>GMQDERWNHPLYTTTAINDEELEGHAYIPGGLKVQTS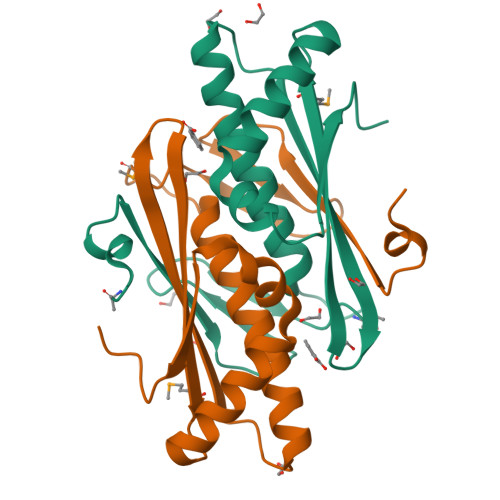SPMNDHPGTNPEQLLGLSLSTCLEATLEAVEKEHGLPHTGAVRVKVAFIGARAEYQFLVHAQVMVKGVDFDTAKAFTNEIENRCPVSKLLKNSGNYTIETVTDFKD[2x]> KM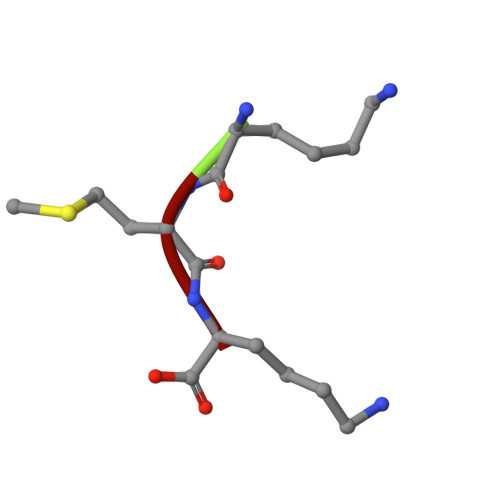K>SNAEDVERATDIVMRQDSADANLVRMGDKHVMFSESGNAFIMYGIQGRSWIAFADPVGDEEDFPDLVWQFVEAARGAGARAAFYQISPFLLSHCADAGLRAFKLGELALVDLTAFELKGGKLATLRQSLSRGARDGLTFEVVEQSQVPDIMDELQQVSDGWLAHHNTREK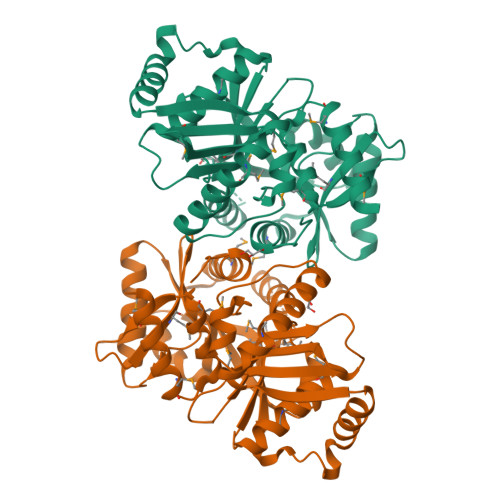RFSLGAFEPDYILSQPVAVLRKDGKITAFANLMVTETKKEATIDLMRFSADAPRGSMDFLFVSIMQHLREAGYESFNLGMAPMSGMSKRDAAPVWDRIGSTLFEHGERFYNFKGLRAFKAKFHPKWEPRYLAVQNGADAALALMDATVLISGGVRGVIGK[6x]> MGHHHHHHGNITLTKRQQEFLLLNGWLQLQCGHAERACILLDALLTLNPEHLAGRRCRLVALLNNNQGERAEKEAQWLISHDPLQAGNWLCLSRAQQLNGDLDKARHAYQHYLELKDHNESP;> GAMGALPPDGHPVEPHLERLYPTAQSKRSLWDFASPGYTFHGLHRAQDYRRELDTLQSLLTTSQSSELQAAAALLKCQQDDDRLLQIILNLLHKV

Several gram-negative bacteria employ type III secretion systems (T3SS) to inject effector proteins into eukaryotic host cells directly from the bacterial cytoplasm. The export gate SctV (YscV in Yersinia) binds substrate:chaperone complexes such as YscX:YscY, which are essential for formation of a functional T3SS. Here, we present structures of the YscX:YscY complex alone and bound to nonameric YscV. YscX binds its chaperone YscY at two distinct sites, resembling the heterotrimeric complex of the T3SS needle subunit with its chaperone and co-chaperone.

In addition to our structure of YscX50:YscY, we also crystallized a longer construct containing residues 32–122 of YscX (YscX32:YscY). Crystallization of this complex required the reductive methylation of primary amines. The resolution was considerably poorer, with the protein adopting a loose packing in space group I4122 with a solvent content of 64.3%. The overall fold is identical to that of the shorter construct and the structures align well with r.m.s.d. values of 2.033 Å between YscX32:YscY and chain A and B of YscX50:YscY or 1.388 Å with chain C and D of the latter. In general, the r.m.s.d. values were a bit higher for YscX (1.489 Å or 1.383 Å for chain B or chain D, respectively) than for YscY (1.233 Å or 1.078 Å) and the models differ the most in the position of the loop between helices α1 and α2 of YscX and in a slightly increased bending at the C-terminus of α3 in the model for YscX32:YscY. Even though this YscX construct is 18 residues longer than YscX50, only L47-P49 of these are resolved, suggesting that the N-terminus is largely disordered. Moreover, the C-terminus in this model is fully resolved and is helical albeit with high B-factors for the last residues. We found that the N-terminal 31 residues of YscX are prone to proteolysis, indicating that they may not exhibit a tertiary structure.> PQPPADEQPEPRTRRRAYLWCKEFLPGAWRGLREDEFHISVIRGGLSNMLFQCSLPDTTATLGDEPRKVLLRLYGAILQMRSCNKEGSEQAQKENEFQGAEAMVLESVMFAILAERSLGPKLYGIFPQGRLEQFIPSRRLDTEELSLPDISAEIAE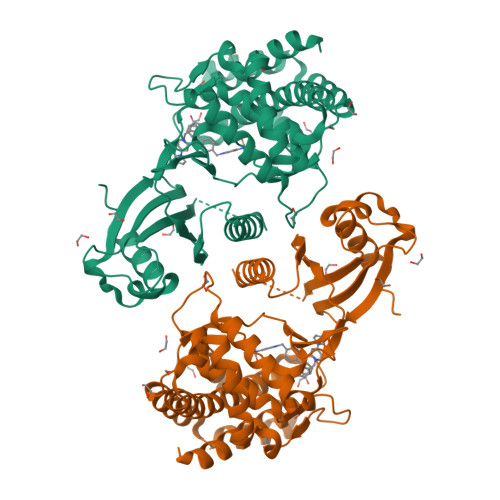KMATFHGMKMPFNKEPKWLFGTMEKYLKEVLRIKFTEESRIKKLHKLLSYNLPLELENLRSLLESTPSPVVFCHNDCQEGNILLLEGRENSEKQKLMLIDFEYSSYNYRGFDIGNHFCEWMYDYSYEKYPFFRANIRKYPTKKQQLHFISSYLPAFQNDFENLSTEEKSIIKEEMLLEVNRFALASHFLWGLWSIVQAKISSIEFGYMDYAQARFDAYFHQKRKLGV Glycogen phosphorylase (GP; EC 2.4.1.1) is the enzyme that catalyzes the first step of glycogenolysis toward the production of glucose-1-phosphate. GP is an allosteric enzyme according to the Wyman–Monod–Changeux model and, through effector binding, adopts two interconverting states, a low-activity (T) state and a high-activity (R) state. GP has several ligand-binding sites that can be exploited for inhibitor binding. The structures of rmGPb-EGCG and rmGPb-EGC complexes were determined by X-ray crystallography, showing binding at the quercetin binding site (QBS) in agreement with kinetic studies that revealed both compounds as noncompetitive inhibitors of GP, with EGCG also causing a significant reduction in cell viability and migration of U87-MG glioblastoma cells.

The 2Fo–Fc map also showed that EGC binds at the QBS although a high concentration of EGC (15 mM, 3× more than EGCG) was needed in order to achieve binding, reflecting its low potency toward GP. In comparison, the Ki value of EGC was calculated to be 285.5 ± 14.1 μΜ for rmGPb and the IC50 value for hlGPa was 193.8 ± 3.5 μM, revealing that the gallate group of EGCG confers potency. EGC forms 22 less van der Waals interactions (overall 85, 7 polar–polar, 37 nonpolar–nonpolar, and 41 polar–nonpolar) compared to EGCG. The lack of the gallate group and its hydroxyls explains differences mostly in polar interactions and also in hb bonding. EGC forms 3 hb with protein residues in comparison to 5 of EGCG. The hydroxyl oxygen O19 of ring A makes 2 water-bridged interactions: the water-bridged interactions O19-Wat1037-Cys495 (O) and the water-bridged interactions O19-Wat1847-Leu494 (O) and the hydrogen-bridged interactions 1 hb with Wat1848. In addition, (O21) forms 1 hb with Wat1103, and the overall EGC forms 8 hb interactions. Arg551 is at a 3.58 Å distance from ring B and Lys544 is at a distance of 3.23 Å from ring A, participating in π–cation interactions. Superposition of the binary complexes of rmGPb-EGCG with rmGPb-EGC reveals a shift (RMSD, 3.31 Å) of the Glu120(OE2) side chain upon EGCG binding due to its hydrogen-bonding interaction with hydroxyl oxygen (O44) of the gallate group.

> QEKRKQISVRGLAGVENVTELKKNFNRHLHFTLVKDRNVATPRDYYFALAHTVRDHLVGRWIRTQQHYYEKDPKRIYYLSLEFYMGRTLQNTMVNLALENACDEATYQLGLDMEELEEIEEDAGLGNGGLGRLAACFLDSMATLGLAAYGYGIRYEFGIFNQKICGGWQMEEADDWLRYGNPWEKARPEFTLPVHFYGRVEHTSQGAKWVDTQVVLAMPYDTPVPGYRNNVVNTMRLWSAKAPNDFNLKDFNVGGYIQAVLDRNLAENISRVLYPNDNFFEGKELRLKQEYFVVAATLQDIIRRFKSSKFGCRDPVRTNFDAFPDKVAIQLNDTHPSLAIPELMRVLVDLERLDWDKAWEVTVKTCAYTNHTVIPEALERWPVHLLETLLPRHLQIIYEINQRFLNRVAAAFPGDVDRLRRMSLVEEGAVKRINMAHLCIAGSHAVNGVARIHSEILKKTIFKDFYELEPHKFQNKTNGITPRRWLVLCNPGLAEIIAERIGEEYISDLDQLRKLLSYVDDEAFIRDVAKVKQENKLKFAAYLEREYKVHINPNSLFDVQVKRIHEYKRQLLNCLHVITLYNRIKKEPNKFVVPRTVMIGGKAAPGYHMAKMIIKLITAIGDVVNHDPVVGDRLRVIFLENYRVSLAEKVIPAADLSEQISTAGTEASGTGNMKFMLNGALTIGTMDGANVEMAEEAGEENFFIFGMRVEDVDRLDQRGYNAQEYYDRIPELRQIIEQLSSGFFSPKQPDLFKDIVNMLMHHDRFKVFADYEEYVKCQERVSALYKNPREWTRMVIRNIATSGKFSSDRTIAQYAREIWGVEPSRQRLP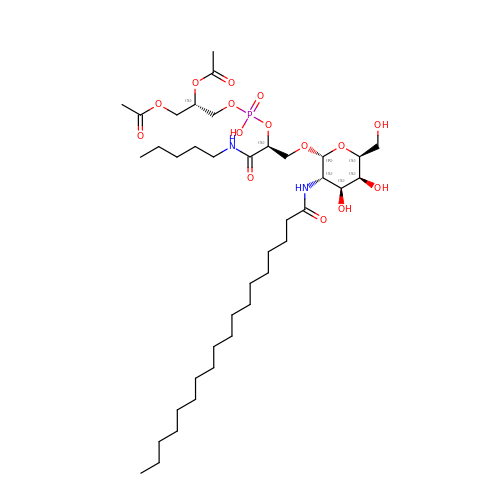[(2~{S})-2-acetyloxy-3-[[(2~{S})-3-[(2~{R},3~{S},4~{S},5~{S},6~{S})-6-(hydroxymethyl)-3-(octadecanoylamino)-4,5-bis(oxidanyl)oxan-2-yl]oxy-1-oxidanylidene-1-(pentylamino)propan-2-yl]oxy-oxidanyl-phosphoryl]oxy-propyl] ethanoate | C39 H73 N2 O15 P | ZPGLDLNPYVCZJR-XTLGHBECSA-N>MTTQQLKEKISKIIDNFSGIRVVFTTTANELKLSRIEGSALNSIAEGFIDKIKEDIINNEDLTSPLLSNFDDRKNALFKFDYEQYPEEFNKITQAIAIPPNSQDYYNPLNKFTDVKGIIILISGDNKCLALYKNKTNLAVLRNSRKMFNLVPDPDGYLKQLPNEILRLDFNYDLFSIGEDFYIKNHKTLETQMKFHQVIEAQAVIALNSLRDSLLIEDISGLEKSSREISFARKLAKISKHSPVLGKIDTKTIIDYVSQHKYLSAILQINE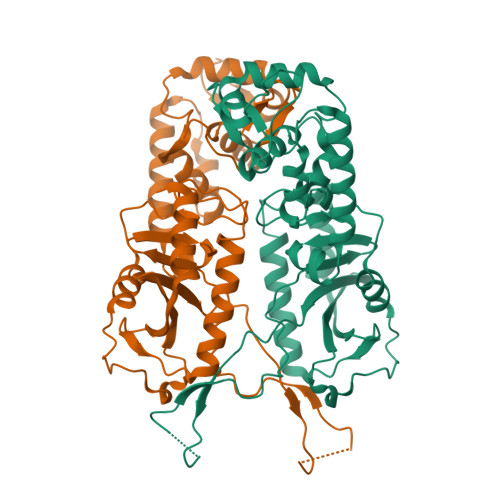AGDKLLIKTKTSQKHFIKLMSDDYLQSDLTKIIYMSIAKDRLDE[2x]> VAFGADAAKTTQEKFDALKEAGVFSAYPGTT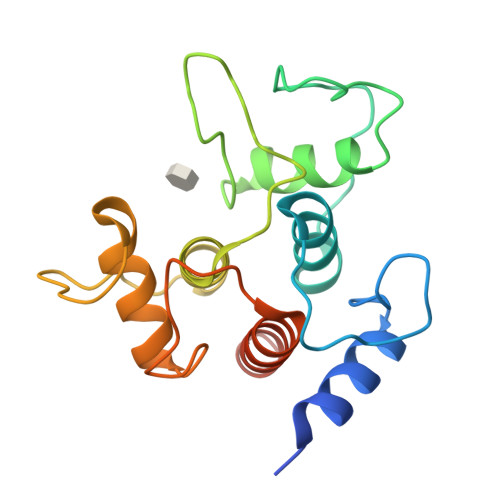DAKLGQDMTRAEFAKVLVKLFGLKEIHGQYSYKDKNYDAKNWAAPFIEAVTAEGLMQAKDLTKKIFDFNGKITVEEASKTLVTALKLEPVKDAQNKATDWAKGYFEAAVNAGLFSKDANPKANATRAQLVEAAFAADEMSKGSGSHHHHHH N-[4-[[3-(2,4-DIAMINO-1,6-DIHYDRO-6-OXO-4-PYRIMIDINYL)-PROPYL]-[2-((2-OXO-2-((4-PHOSPHORIBOXY)-BUTYL)-AMINO)-ETHYL)-THIO-ACETYL]-AMINO]BENZOYL]-1-GLUTAMIC 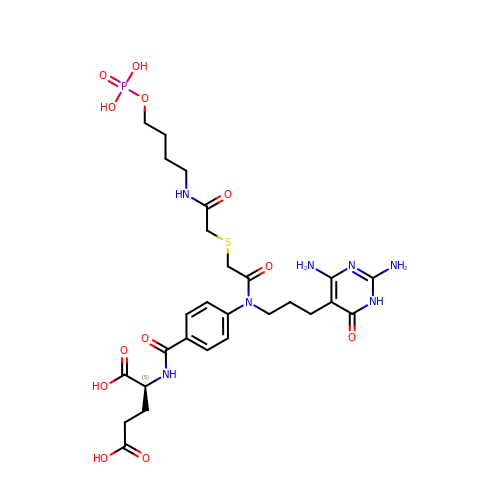ACID | C27 H38 N7 O12 P S | WIBNWPBCQGWSJV-IBGZPJMESA-N>MSKTVEEIWAAQRARGPATVLAIGTAAPANVVYQADYPDYYFRITKSEHMTELKEKFRRMCDKSMITKRHMHLSEELLKNNPDICAYMAPSLDARQDMVVVEVPKLGKEAAAKAIKEWGRPKSAITHLIFCTTSGVDMPGADFQLTKLLGLCPSVRRTMLYQQGCFAGGTVLRLAKDLAENNAGARVLVVCSEITAVTFRGPSETHLDSMVGQALFGDGASAIIVGADPDPVIERPLFQIVSAAQTILPDSDGAIDGHLREVGLTFHLLKDVPGLISKNIEKSLKEAFAPLGIDDWNSIFWIVHPGGPAILDQ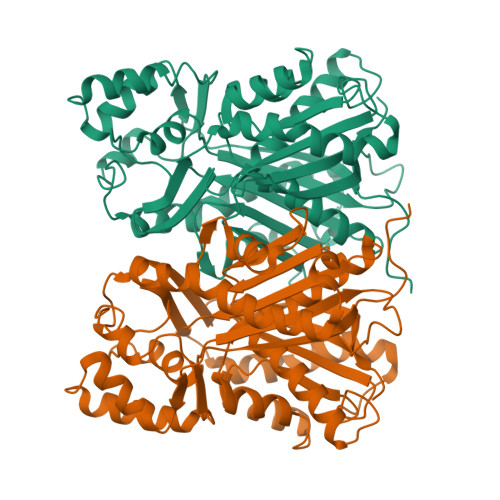VEAKLRLKVEKLKTTRTVLSEYGNMSSACVLFILDEMRRNSMEEGKATTGEGLHWGVLFGFGPGLTVETVVLHSLPIAEAN[2x]> MSGQSLTDRITAAQH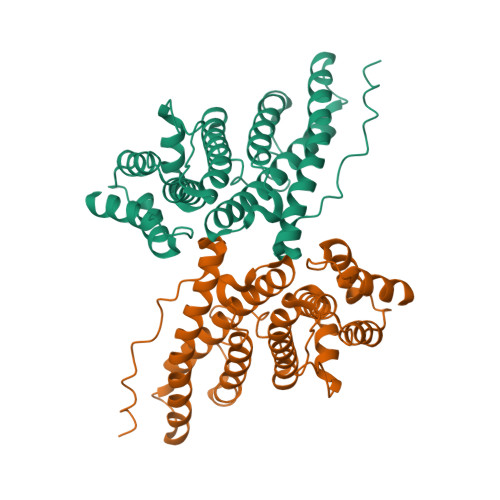SVTGSAVSKTVCKATTHEIMGPKKKHLDYLIQCTNEMNVNIPQLADSLFERTTNSSWVVVFKSLITTHHLMVYGNERFIQYLASRNTLFNLSNFLDKSGLQGYDMSTFIRRYSRYLNEKAVSYRQVAFDFTKVKRGADGVMRTMNTEKLLKTVPIIQNQMDALLDFNVNSNELTNGVINAAFMLLFKDAIRLFAAYNEGIINLLEKYFDMKKNQCKEGLDIYKKFLTRMTRISEFLKVAEQVGIDRGDIPDLSQAPSSLLDALEQHLASLEGKK>[3x]MNKQNFLQTGGFPLETDTLNAMQEAYSVFNALGELAGNKAIIKGCVVSGSTTT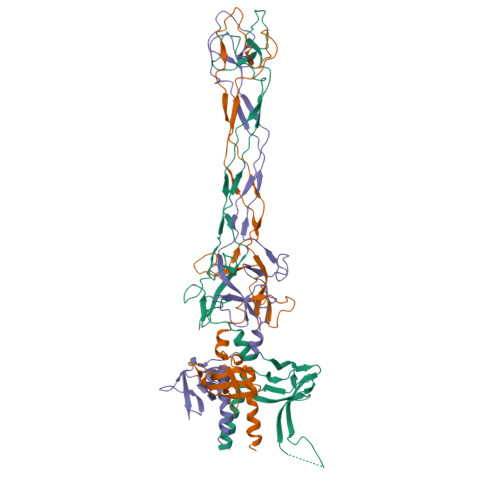DGVVYINGEVFKFVGGQTQSRVKILETSTSKEFEDGSTNAVHFERYVTFASGTGSISWAEFAKLTTLRELSRRLLPAGTNPQLYSGSVNNIPSGWQLCDGTNGTENLKGSFIVGYDPNDSDYNAIGKVGGTKKVTPSGNLDSRSINVTVPRDGWSTFGSGLGAVKSGRIVVGSGQQENSEYLESLRASGIDRTLTSTPHSHTFTGNQQDNRAPYYTLAYIIYIG>RKCSLTGKWTNDLGSNMTIGAVNSRGEFTGTYTTAVTATSNEIKESPLHGTENTINKRTQPTFGFTVNWKFSESTTVFTGQCFIDRNGKEVLKTMWLLRSSV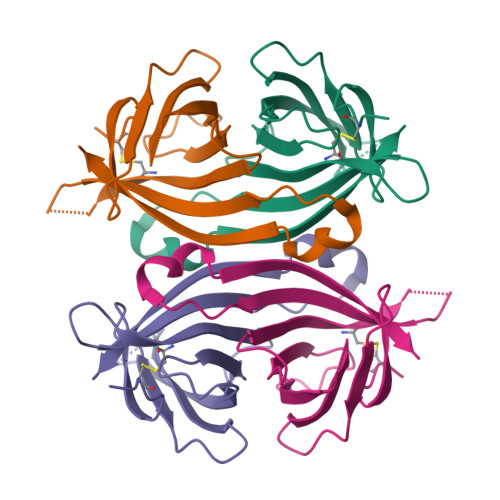NDIGDDKKATRVGINIFTRL[2x]> MKTFFLIVHTIISVALIYMVQVQMSKFSELGGAFGSGGLH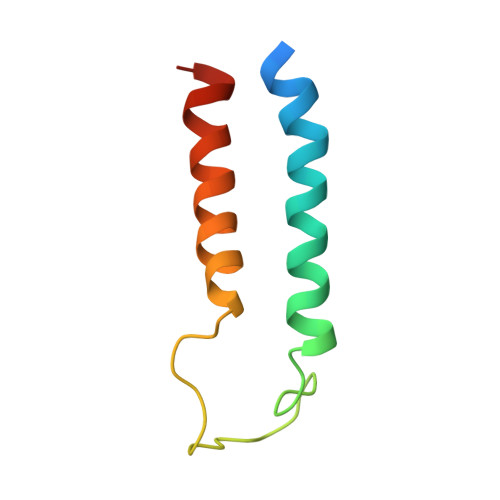TVFGRRKGLDTGGKITLVLSVLFFVSCVVTAFVLTR>MLDELVKKELSEEEITEIKLEEIIKYITLIKKSKTFVSSEIRKEELKFLSELAESLFELRLSKVLEGKVGKGFDEFIFDIFKILKQFYVDLLTGRYIIYNDKIYCIVQKPLIYNDHRVNEGDVLVLPMREALPLIIASYLTPYKIDIEEQL[2x];>MIEVKLRAIKRLSNVYTRRVMIIEDWNGS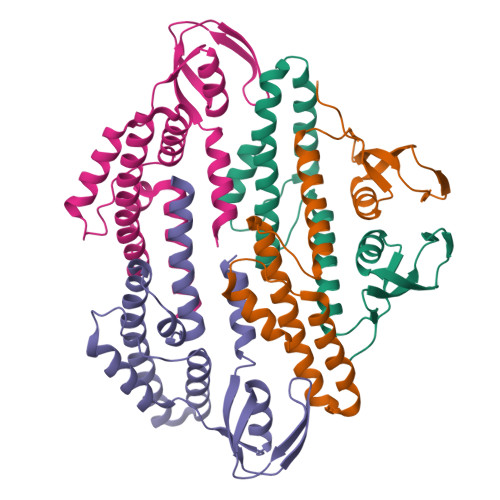SITTGNIELVKGSENQLPQWLAIILEGKKVAKIEDKISIEDLGRILFQERQNMNTPASLVPLGKDFTSRVQLYLETLRKDNNVESLEKLRKSIGILNEIIKIRLRKLIQLAFLNIDDQNLINGMTEEELLIYKTIKQLIKELYGDIIGNS[2x]> GGPMGNGMNKILPGLYIGNFKDARDAAQLSANAVTHILSVHDSARPMLEGVKYLCIPAADSPSQNLTRHFKESIKFIHECRLRGESCLVHSLAGVSRSVTLVIAYIMTVTDFGWEDALHTVRAGRSCANPNVGFQRQLQEFEKHEVHQYRQW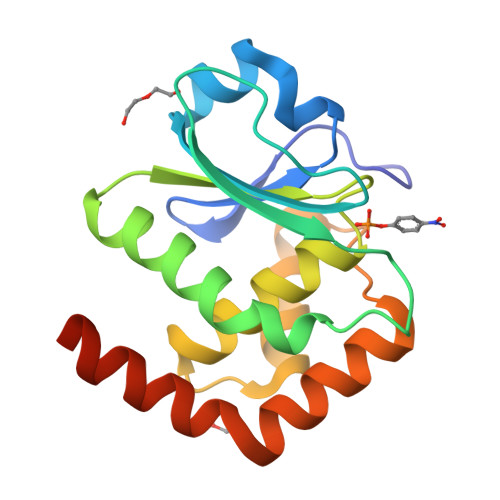LKEEYGESPLQDAE>[2x]MQYDDDCKLARGGPPATIVAIDEESRNGTILVDNMLIKGTAGGPDPTIELSLKDNVDYWVLLDPVKQMLFLNSTGRVLDRDPPMNIHSIVVQVQCVNKKVGTVIYHEVRIVVRDRNDNSPTFKHESYYATVNELTPVGTTIFTGFSGDNGATDIDDGPNGQIEYVIQYNPEDPTSNDTFEIPLMLTGNVVLRKRLNY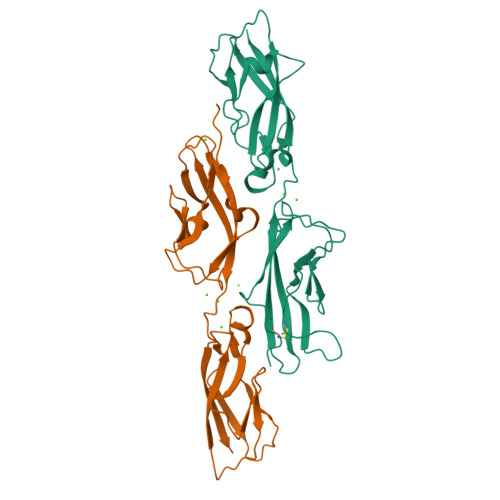EDKTRYYVIIQANDRAQNLNERRTTTTTLTVDLEHHHHHH;>MQVNRLPFFTNHFFDTYLLISEDTPVGSSVTQLLARDMDNDPLVFGVSGEEASRFFAVEPDTGVVWLRQPLDRETKSEFTVEFSVSDHQGVITRKVNIQVGDVNDNAPTFHNQPYSVRIPENTPVGTPIFIVNATDPDLGAGGSVLYSFQPPSPFFAIDSARGIVTVIQELDYEVTQAYQLTVNATDQDKTRPLSTLANLAIIITDLEHHHHHH[2x]>[2x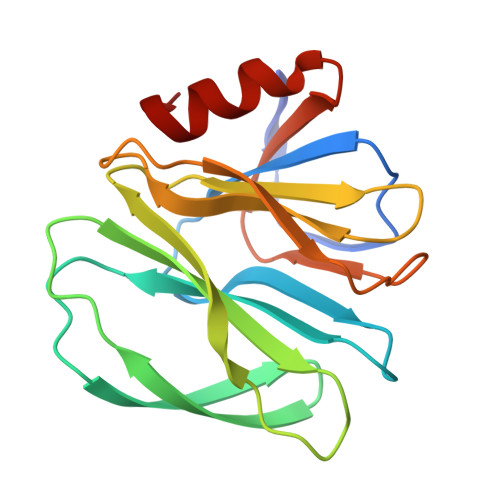]GSALDGPYTPDSSNLPSNYWYLINPLNDGVVFSVTNNSTFWMFTYLILPNTAQTNVTVNVMNETVNISIDNSGSTYRFVDYFKTSSTQSYRQRNYLITEHRLQAYRRDESGNISNYWGSSTYGDLRVGTYFNPVLNAVINLNADFYIIPDSQQEKCTEYIKGGL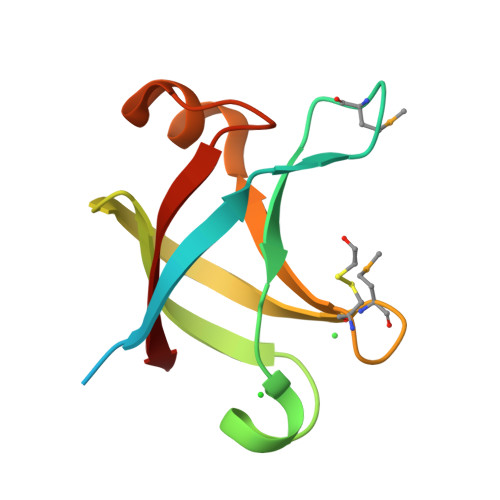> MKKTLPKTEAPSSVGNGSDSPIEFDAIIRQVPDMDAAYVEIPFDVKTVYGKGRVRVNATFDGYPYTGYIVRMGLPCHILGLRQDIRRAIGKQPGDSVYVTLLPL>[5x]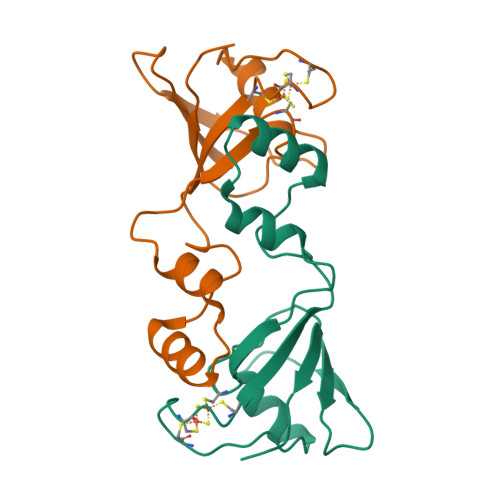MATIYFSSPLMPHNKKVQAVAGKRSTLLGVAQENGVKIPFECQDGNCGSCLVKITHLDGERIKGMLLTDKERNVLKSVGKLPKSEEERAAVRDLPPTYRLACQTIVTDEDLLVEFTGEPGGA>[2x]MAHHHHHHMKLLVIGNGGREHALAWKLAQSPKVETVFVAPGNAGTAIESKLQNIALTAYQDLIEFCRKENIVFTVVG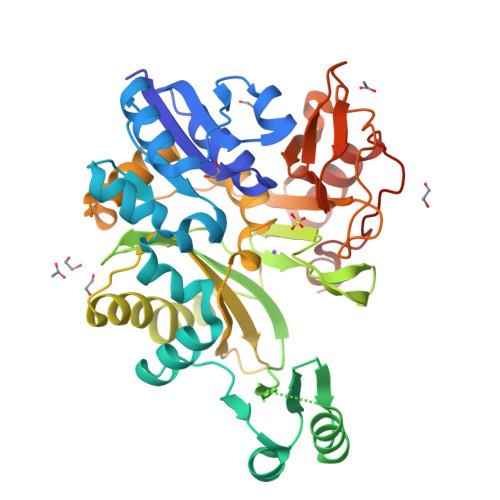PEAPLAAGIVDDFRAAGLKIFGPTQYAAQLESSKDFAKAFMVKYNIPTAQYQTFENADAAHDYVNQKGAPIVIKADGLVAGKGVIVAMTLDEAHAAIDDMLLGNKMGNAGERVVIEDFLQGEEASFIVMVDGNHVLPMATSQDHKRLLDGDKGPNTGGMGAYSPAPVVTPAVYERAMNEIILPTVAGMKAEGHEFTGFLYAGLMIDQSGAPYTIEFNCRFGDPETQPIMSRLNSDLADLVEAAIDGRLDSVKAEWNPQTAVGVVLAAQNYPETPKKGDVISGLDDVNRIGKVFHAGTTVNEKGDVLTNGGRILCVVGLGDDVAQAKAKAYGALEKISFDGMQYRKDIADKAINR>MMIVYKGEKMQFIRVNTLKINPEVLKKRLENKGVVLEKTFLDYAFEVKKSPFSIGSTPEYLFGYYMPQSISSMIPPIVLNPREDDFILDMCAAPGGKTTHLAQLMKNKGTIVAVEISKTRTKALKSNINRMGVLNTIIINADMRKYKDYLLKNEIFFDKILL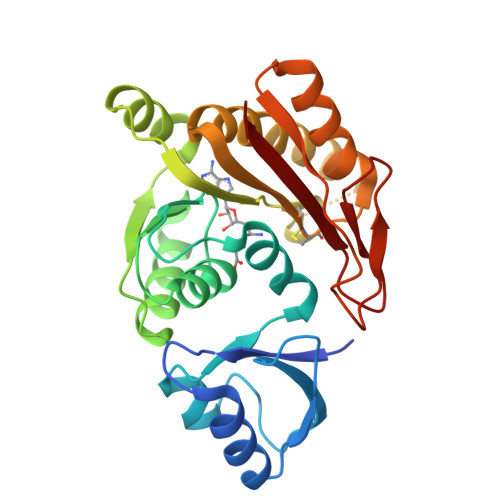DAPCSGNIIKDKNRNVSEEDIKYCSLRQKELIDIGIDLLKKDGELVYSTCSMEVEENEEVIKYILQKRNDVELIIIKANEFKGINIKEGYIKGTLRVFPPNEPFFIAKLRKI[2x]>MESPSSEEEKPLAKMAFTLADRVTEEMLADKAALVVEVVEENYHDAPIVGIAVVNEHGRFFLRPETALADPQFVAWLGDETKKKSMFDSKRAAVALKWKGIELCGVSFDLLLAAYLLDPAQGVDDVAAAAKMKQYEAVRPDEAVYGKGAKRAVPDEPVLAEHLVRKAAAIWELERPFLDELRRNEQDRLLVELEQPLSSILAEMEFAGVKVDTKRL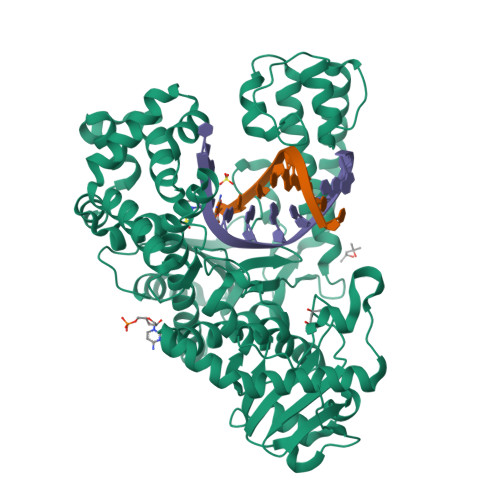EQMGKELAEQLGTVEQRIYELAGQEFNINSPKQLGVILFEKLQLPVLKKTKTGYSTSADVLEKLAPYHEIVENILHYRQLGKLQSTYIEGLLKVVRPATKKVHTIFNQALTQTGRLSSTEPNLQNIPIRLEEGRKIRQAFVPSESDWLIFAADYSQIALRVLAHIAEDDNLMEAFRRDLDIHTKTAMDIFQVSEDEVTPNMRRQAKAVNFGIVYGISDYGLAQNLNISRKEAAEFIERYFESFPGVKRYMENIVQEAKQKGYVTTLLHRRRYLPDITSRNFNVRSFAERMAMNTPIQGSAADIIKKAMIDLNARLKEERLQAHLLLQVHDELILEAPKEEMERLCRLVPEVMEQAVTLRVPLKVDYHYGSTWYDAK[2x]>MASWSHPQFEKGAVTSLYKKAGFKDLTMLLDELKDMSFFNKGDICLIGCSTSEVIGEKIGTVGSMEVAETIFNALDVVSKETGVTFAFQGCEHINRAITIEKSQYNPLTMEEVSVVPDVHAGGSLATYAFQHMKDPIVVEHITVPCGIDIGQTLIGMHI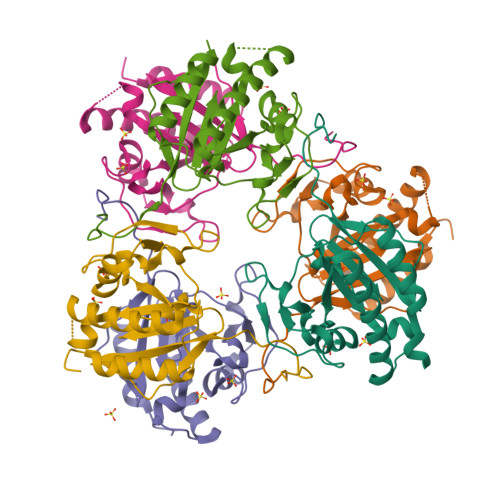KHVCVPVRTSVKQVGQAIVTIATSRPKKIGGERAKYQ[6x]Methylation of cytosine 32 in the anticodon loop of tRNAs to 3-methylcytosine (m3C) is crucial for cellular translation fidelity. Here, we report the cryo-electron microscopy structure of the human m3C tRNA methyltransferase METTL6 in complex with seryl-tRNA synthetase (SerRS) and their common substrate tRNASer. We show that SerRS acts as the tRNASer substrate selection factor for METTL6. We demonstrate that SerRS augments the methylation activity of METTL6 and that direct contacts between METTL6 and SerRS are necessary for efficient tRNASer methylation.

Therefore, for the purpose of structure determination, we stabilized the assembly by fusing METTL6 to the flexible C terminus of SerRS and coexpressed both proteins as a single polypeptide in insect cells. Processing of the cryo-EM micrographs and particle images of the METTL6–SerRS–tRNASer complex revealed three-dimensional (3D) classes for 1:2:1, 1:2:2 and 2:2:2 stoichiometries with essentially identical intermolecular contacts in the METTL6–SerRS–tRNA interface. In brief, at the core of the 1:2:2 METTL6–SerRS–tRNA complex, two molecules of tRNASer bind symmetrically across the SerRS dimer without contact with each other. Each tRNASer interacts with both SerRS protomers. METTL6 is located at the extremity of the complex, binding its proximal tRNASer anticodon stem and the variable arm that protrudes from the SerRS–tRNASer complex. The tRNASer long variable arm is coordinated in the interface between METTL6 and the SerRS N-terminal stalk. In the same interface, two protein loops of SerRS interact directly with METTL6. Comparing the METTL6-bound tRNASer to the METTL6-unbound tRNASer copy in our structure, and also to free tRNA, we observe extensive remodeling of the anticodon arm and its global bending toward METTL6. Strikingly, in the complex structure, this C32-A38 base pair is disrupted and the bases are flipped to the outside of the anticodon loop.

> MASLQRKGLQARILTSEEEEKLKRDQTLVSDFKQQKLEQEAQKNWDLFYKRNSTNFFKDRHWTTREFEELRSCREFEDQKLTMLEAGCGVGNCLFPLLEEDPNIFAYACDFSPRAIEYVKQNPLYDTERCKVFQCDLTKDDLLDHVPPESVDVVMLIFVLSAVHPDKMHLVLQNIYKVLKPGKSVLFRDYGLYDHAMLRFKASSKLGENFYVRQDGTRSYFFTDDFLAQLFMDTGYEEVVNEYVFRETVNKKEGLCVPRVFLQSKFLKPPKNPSPVVLGLDPKS;>[2x]MVLDLDLFRVDKGGDPALIRETQEKRFKDPGLVDQLVKADSEWRRCRFRADNLNKLKNLCSKTIGEKMKKKEPVGDDESVPENVLSFDDLTADALANLKVSQIKKVRLLIDEAILKCDAERIKLEAERFENLREIGNLLHPSVPISNDEDVDNKVERIWGDCTVRKKYSHVDLVVMVDGFEGEKGAVVAGSRGYFLKGVLVFLEQALIQYALRTLGSRGYIPIYTPFFMRKEVMQEVAQLSQFDEELYKVIGKGSEKSDDNSYDEKYLIATSEQPIAALHRDEWLRPEDLPIKYAGLSTCFRQEVGSHGRDTRGIFRVHQFEKIEQFVYSSPHDNKSWEMFEEMITTAEEFYQSLGIPYHIVNIVSGSLNHAASKKLDLEAWFPGSGAFRELVSCSNCTDYQARRLRIRYGQTKKMMDKVEFVHMLNATMCATTRTICAILENYQTEKGITVPEKLKEFMPPGLQELIPFVKPAPIEQEPSKKQKKQHEGSKKKAAARDVTLENRLQNMEVTDA> EEVRQFRRLFAQLAGDDMEVSATELMNILNKVVTRHPDLKTDGFGIDTCRSMVAVMDSDTTGKLGFEEFKYLWNNIKKWQAIYKQFDVD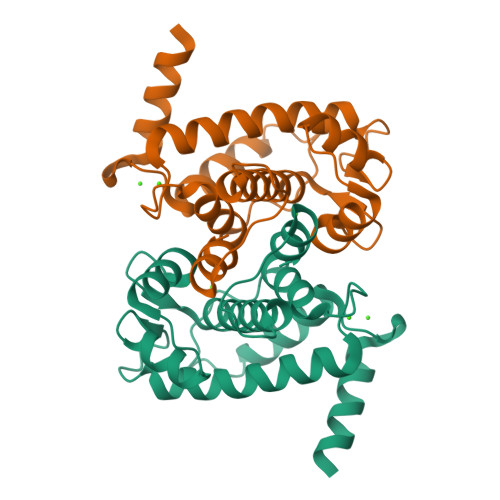RSGTIGSSELPGAFEAAGFHLNEHLYSMIIRRYSDEGGNMDFDNFISCLVRLDAMFRAFKSLDKDGTGQIQVNIQEWLQLTMYS> VAM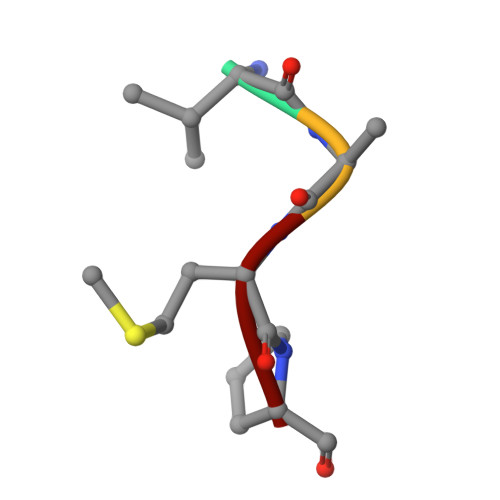P> MSDPS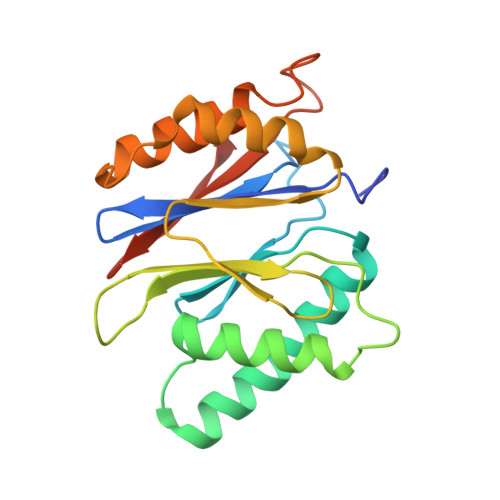SINGGIVVAMTGKDCVAIACDLRLGSQSLGVSNKFEKIFHYGHVFLGITGLATDVTTLNEMFRYKTNLYKLKEERAIEPETFTQLVSSSLYERRFGPYFVGPVVAGINSKSGKPFIAGFDLIGCIDEAKDFIVSGTASDQLFGMCESLYEPNLEPEDLFETISQALLNAADRDALSGWGAVVYIIKKDEVVKRYLKMRQD>MAPLATRQGKRPSKNLKARCSRKALHVNFKDMGWDDWIIAPLEYEAFHCEGLCEFPLRSHLEPTNHAVIQTLMNSMDPESTPPTCCVPTRLSPISILFIDSANNVVYKQYEDMVVESCGCR[2x];>ETGCNKALCASDVSKCLIQELCQCRPGEGNCSCCKECMLCLGALWDECCDCVGMCNPRNYSGTLEVLFQ[2x]

Twisted gastrulation (TWSG1) is an evolutionarily conserved secreted glycoprotein which controls signaling by Bone Morphogenetic Proteins (BMPs). TWSG1 binds BMPs and their antagonist Chordin to control BMP signaling during embryonic development, kidney regeneration and cancer. TWSG1 is composed of two distinct, disulfide-rich domains. The TWSG1 N-terminal domain occupies the BMP type 1 receptor binding site on BMPs, whereas the C-terminal domain binds to a Chordin family member.

Serendipitously, the TWSG1–GDF5 complex crystallized in the presence of CaCl2, and we identified a calcium-binding site that mediated TWSG1–GDF5 interactions at the periphery of the binding interface. Unexpectedly, the structure of the TWSG1–GDF5 complex reveals a previously unknown calcium-binding site at the edge of TWSG1–GDF5 interface. We confirmed the identity of the calcium ions by anomalous difference Fourier analysis. The calcium ion is coordinated by 8 oxygen atoms with an average distance of 2.55 Å: carboxyl group of GDF5 Asp416, main-chain carbonyl oxygen of GDF5 Gly413 and 5 water molecules. 2 out of 5 water molecules bridge the calcium ion to the carboxyl group of TWSG1 Asp34. The calcium-binding site is stabilized by a hydrogen bond between TWSG1 Ser33 and GDF5 Trp414, and other interactions (salt bridge between TWSG1 Asp34 and Lys37; T-shaped π-π stacking of Trp414 and Trp417 of GDF5). The mutation of the calcium-binding residue Asp34 to Ala in TWSG1 did not abolish the TWSG1–BMP interactions, indicating a minor regulatory role for calcium. Since the calcium-binding residues in BMP ligands are conserved, and calcium is ubiquitously present in the extracellular space, our TWSG1–GDF5 structure brings this ion into focus.>[2x]MSLQTCVLHRLSLPLKFPMRTAHGHIREKQAILVQLVDADGIEGWSECVALAEPTYTEECTDTAWVMLVHHLV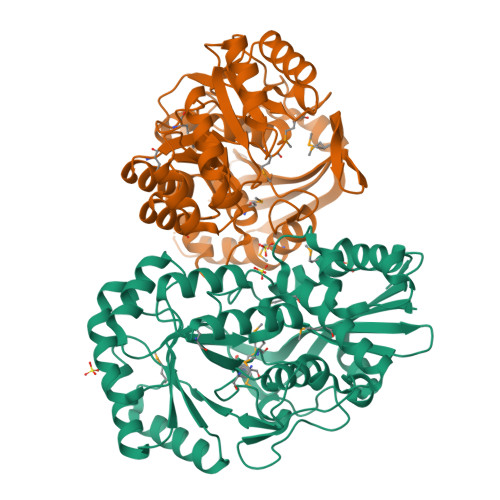PRFARWLRAASQDQDVDPRTVCEALRDVRGNRMSVAAIEMAVWDWYAARTGQPLVGLLGGGRDRVEVSATLGMSESLDVLIQSVDAAVEQGFRRVKLKIAPGRDRAAIKAVRLRYPDLAIAADANGSYRPEDAPVLRQLDAYDLQFIEQPLPEDDWFDLAKLQASLRTPVCLDESVRSVRELKLTARLGAARVLNVKPGRLGGFGATLRALDVAGEAGMAAWVGGMYETGVGRVHGLIAAALPLMRYATDLGPSDRYFEQDVLKEPIAFVEPGVIQVPQCAGVADWVDRDAVRRFSTATWSVDLRTLEGHHHHHH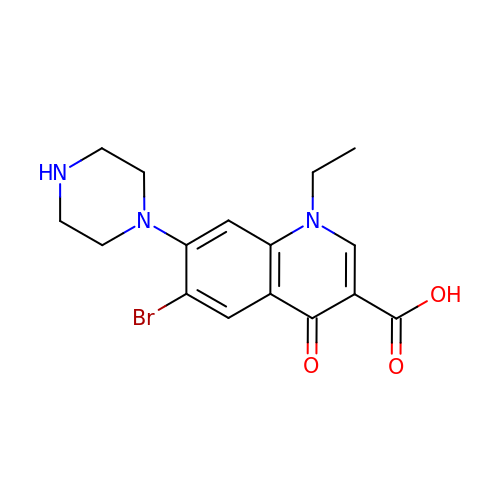6-bromo-1-ethyl-4-oxo-7-(piperazin-1-yl)-1,4-dihydroquinoline-3-carboxylic acid | C16 H18 Br N3 O3 | DAPHRWWQHCSXBW-UHFFFAOYSA-N>[4x]AQCSVDIQGNDQMQFNTNAITVDKSCKQFTVNLS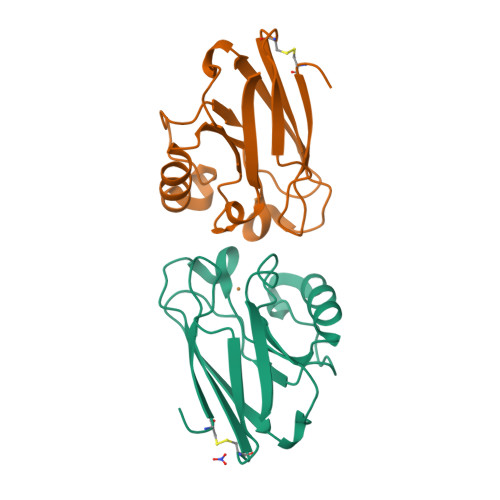LPGNLPKNVMGHNWVLSTAADMQGVVTDGMASGLDKDYLKPDDSRVIAHTKLIGSGEKDSVTFDVSKLKEGEQYMFFCTFPGHSALMKGTLTLK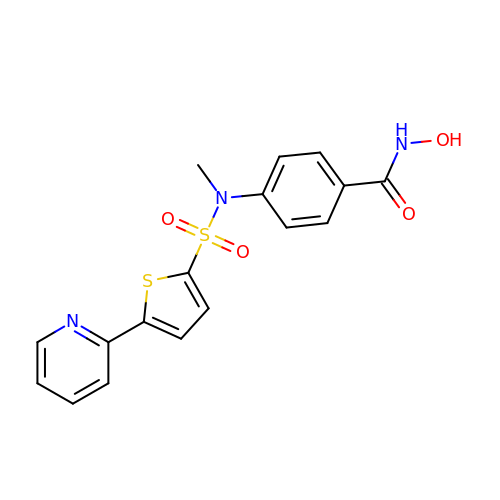N-HYDROXY-4-(METHYL{[5-(2-PYRIDINYL)-2-THIENYL]SULFONYL}AMINO)BENZAMIDE | C17 H15 N3 O4 S2 | LFGYSFPVLMPUPE-UHFFFAOYSA-N>[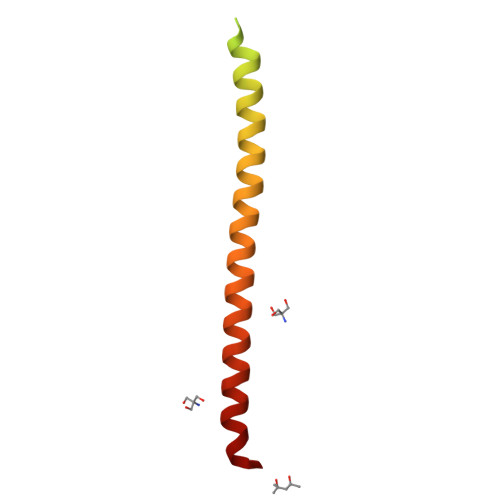2x]GSHMSHLDNTMAIRLLPLPVRAQLCAHLDALDVWQQLATAVKLYPDQVEQISSQKQRGRSASNEFLNIWGGQYNHTVQTLFALFKKLKLHNAMRLIKDYVSEDLHKYI> AVKYYTLEEIQKHNNSKSTWLILHYKVYDLTKYLE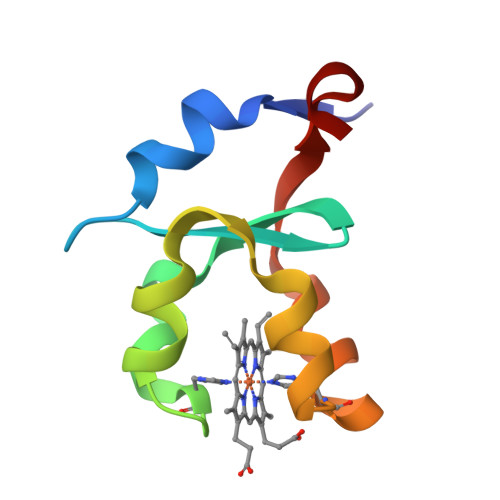EHPGGEEVLREQAGGDATENFEDVGHSTDARELSKTFIIGELHPDDR> GNAKNKESPTKAIVRLREHINLLSKKQSHLRTQITNQENEARIFLTKGNKVMAKNALKKKKTIEQLLSKVEGTMESMEQQLFSIESANLNLETMRAMQEGAKAMKTIHSGLDIDKVDETMDEIREQVELGDEISDAISRP

The endosomal sorting complexes required for transport (ESCRTs) are membrane remodeling machinery that mediate diverse fundamental cellular processes, including the biogenesis of multivesicular body (MVB) during receptor down-regulation, enveloped virus budding, cytokinesis, plasma membrane repair, nuclear pore complex assembly, and nuclear envelope reformation. ESCRT-III is a unique protein complex in that it is metastable and conformationally dynamic, forming hetero-oligomeric filaments of multiple subunits on membranes. Vps20 nucleates the homo-oligomerization of the most abundant ESCRT-III subunit, Snf7, which then recruits Vps24 and Vps2. We then crystallized and solved X-ray crystal structures of Snf7core in two conformations at 1.6 Å and 2.4 Å resolutions, respectively.

When we superimposed our Snf7 structure with available ESCRT-III structures, we were surprised to note that Snf7core does not fold into four α-helices, but instead, it contains only three α-helices that pack into a highly elongated structure. Although the α1/2 hairpin is relatively unchanged, α3 and α4 undergo large-scale structural rearrangements from the proposed autoinhibited ESCRT-III fold. α2 extends into a ~90 Å long α-helix combining the α2 and α3 segments that were distinct α-helices in previously defined ESCRT-III structures. The angle of the flexible loop between α3 and α4 also changes, which enables α4 to position in different orientations relative to the α1-3 hairpin. Comparison of our Snf7core crystal structures we determined revealed two distinct conformations. Although both structures exhibit an open conformation, we noted two different orientations of α4 with respect to the α1/2 hairpin. In open conformation A, α4 extends in the protofilament plane, whereas in open conformation B, α4 is positioned perpendicular to the protofilament plane. Superimposing the two conformations revealed that α4 can rotate by at least ~90° along the axis of the α2/3 helix. Despite the large differences in α4 positioning, α4 makes a similar interaction with the α1/2 hairpin of a Snf7 protomer in a neighboring protofilament in both structures. The L121P mutant exhibited a MVB sorting efficiency of 32%, compared to that of the α1/2 loop residue Asn59 mutant N59P of 75%, suggesting that the α3/4 loop functions as an important flexible 'hinge' that may facilitate different architectural stages of Snf7 polymers.>[2x]GSAKDPMEKFIKQFSFIALENIFRELPNKITHSFNDINDIKPPKLMYPIFYGSYDWHSSVHSHWLLVKILKDFSHFAPKDEIIKALDSQ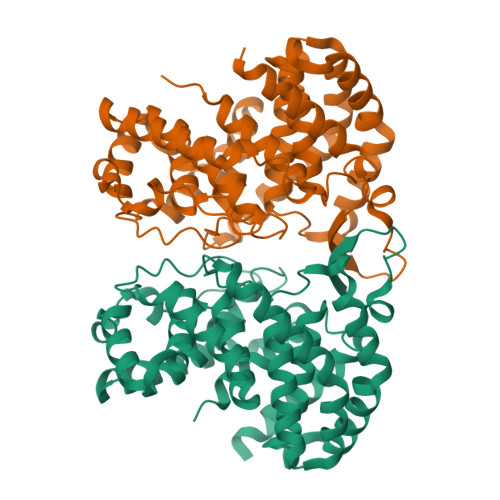FSKEKAEGELKYLQNPAHKGFERPYGWGWFLKLTLEINLLAKENDKAEIWAKNLEGIADFFVKEFKEFLPKMDYPIRVGTHFNSSFALYFALEYARFKKDQELEYCIIQSAKKWFLSDKNMQALEPCGDEFLSPVLMEAVLLSAVLHKNDFVKFFKAYLPNLEAKEPATLFTPVSVSDRSDGKIAHLDGLNLSRAWCFKILSNFCDENLKILLRNNATEHFDKAIAHIEDDYLGSHWLGSFALLALDVDIL Dabrafenib | C23 H20 F3 N5 O2 S2 | 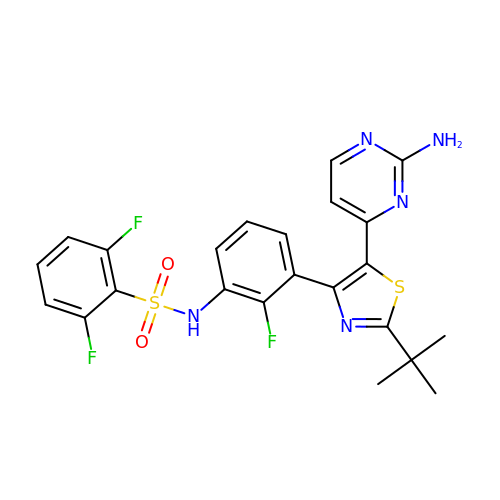BFSMGDJOXZAERB-UHFFFAOYSA-N> MPFTIDSARGIFPNTLAADVVPATIARFSQLNAEDQLALIWFAYLEMGKTLTIAAPGAASMQLAENALKEIQAMGPLQQTQAMCDLANRADTPLCRTYASWSPNIKLGFWYRLGELMEQGFVAPIPAGYQLSANANAVL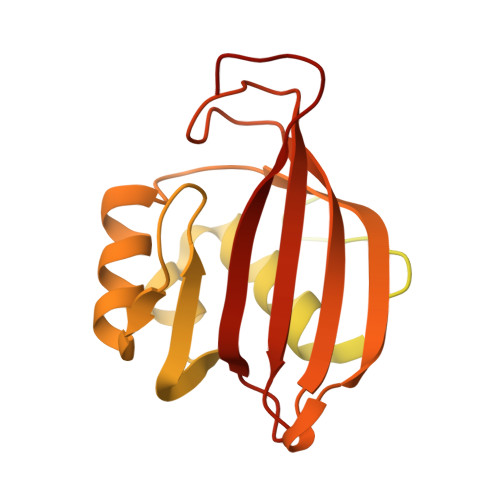ATIQGLESGQQITVLRNAVVDMGFTAGKDGKRIAEPVVPPQDTASRTKVSIEGVTNATVLNYMDNLNANDFDTLIELFTSDGALQPPFQRPIVGKENVLRFFREECQNLKLIPERGVTEPAEDGFTQIKVTGKVQTPWFGGNVGMNIAWRFLLNPEGKIFFVAIDLLASPKELLNFAR>GSMDVVDPDIFNRDPRDHYDLLQRLGGGTYGEVFKARDKVSGDLVALKMVKMEPDDDVSTLQKEILILKTCRHANIVAYHGSYLWLQKLWICMEFCGAGSLQDIYQVTGSLSELQISYVCREVLQGLAYLHSQKKIHRDIKGANILINDAGEVRLADFGISAQIGAELARRLEFIGTPYWMAPEVAAVALKGGYNELCDIWSLGITAIELAELQPPLFDVHPLRVLFLMTKSGYQPPRLKEKGKWSAAFHNFIKVTLTKSP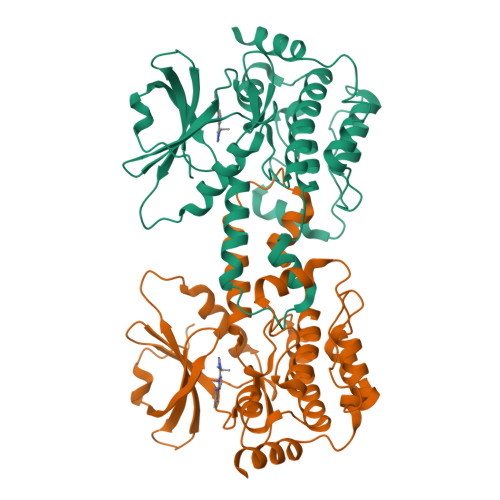KKRPSATKMLSHQLVSQPGLNRGLILDLLDKLKNPGKGPSIGDIEDEE[2x]> MTIRNQRFSLLKQPISSTLNQHLVDYPTPSNLSYWWGFGSLAGICLVIQIVTGVFLAMHYTPHVDLAFNSVEHIMRDVEGGWLLRYMHANGASMFFIVVYLHIFRGLYYASYSSPREF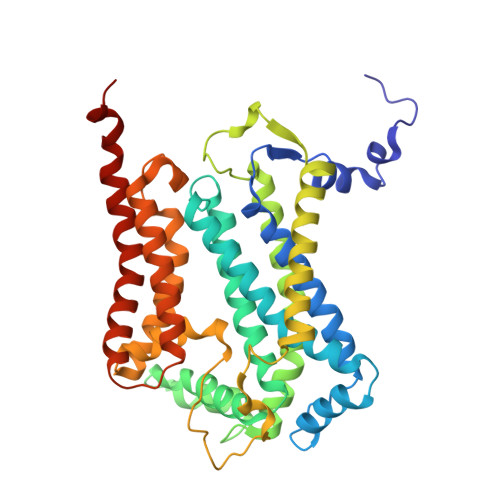VWCLGVVIFLLMIVTAFIGYVLPWGQMSFWGATVITSLASAIPVVGDTIVTWLWGGFSVDNATLNRFFSLHYLLPFILVGASLLHLAALHQYGSNNPLGVHSEMDKIAFYPYFYVKDLVGWVAFAIFFSIWIFYAPNVLGHPDNYIPANPMSTPPHIVPEWYFLPIYAILRSIPDKAGGVAAIALVFICLLALPFFKSMYVRSSSFRPIYQGMFWLLLADCLLLGWIGCQPVEAPFVTIGQISSLVFFLFFAITPILGRVGRGIPNSYTDETDHT> VKDTYTDRLDDWNGIIAGNQYYDSKNDQMAKLNQELEGKVADSLSSISSQADRIYLWEKFSNYKTSANLTATYRKLEEMAKQVTNPSSRYYQDETVVRTVRDSMEWMHKHVYNSEKSIVGNWADYEIGTPRAINNTLSLMKEYFSDEEIKKYTDVIEKFVPDPEHFRKTTDNPFKALGGNLVDMGRVKVIAGLLRKDDQEISSTIRSIEQVFKLVDQGEGFYQDGSYIDHTNVAYTGAYGNVLIDGLSQLLPVIQKTKNPIDKDKMQTMYHWIDKSFAPLLVNGELMDMSRGRSISRANSEGHVAAVEVLRGIHRIADMSEGETKQRLQSLVKTIVQSDSYYDVFKNLKTYKDISLMQSLLSDAGVASVPRTSYLSAFNKMDKTAMYNAEKGFGFGLSLFSSRTLNYEHMNKENKRGWYTSDGMFYLYNGDLSHYSDGYWPTVNPYKMPGTTETDAKRADSDTGKVLPSAFVGTSKLDDANATATMDFTNWNQTLTAHKSWFMLKDKIA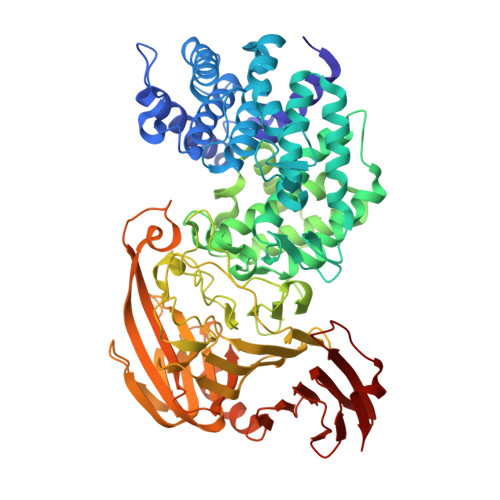FLGSNIQNTSTDTAATTIDQRKLESSNPYKVYVNDKEASLTEQEKDYPETQSVFLESSDSKKNIGYFFFKKSSISMSKALQKGAWKDINEGQSDKEVENEFLTISQAHKQNGDSYGYMLIPNVDRATFNQMIKELESSLIENNETLQSVYDAKQGVWGIVKYDDSVSTISNQFQVLKRGVYTIRKEGDEYKIAYYNPETQESAPDQEVFKKL[(7R,9aR)-7-(4-chlorophenyl)-1,3,4,6,7,8,9,9a-octahydropyrido[1,2-a]pyrazin-2-yl]-(2-bromanyl-3-methoxy-phenyl)methanone 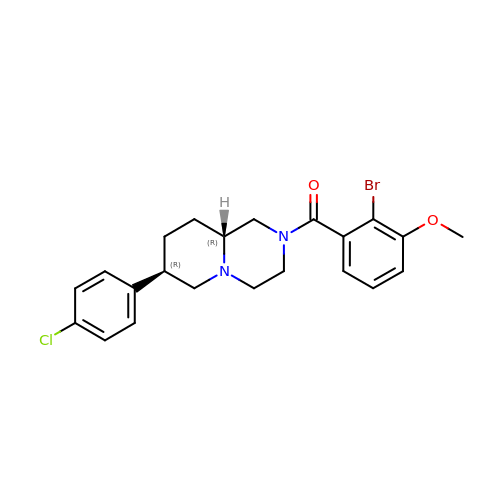| C22 H24 Br Cl N2 O2 | BKTASVDLNMGMFP-FUHWJXTLSA-N> SRKTYTLTDYLKNTYRLKLYSLRWISDHEYLYKQENNILVFNAEYGNSSVFLENSTFDEFGHSINDYSISPDGQFILLEYNYVKQWRHSYTASYDIYDLNKRQLITEERIPNNTQWVTWSPVGHKLAYVWNNDIYVKIEPNLPSYRITWTGKEDIIYNGITDWVYEEEVFSAYSALWWSPNGTFLAYAQFNDTEVPLIEYSFYSDESLQYPKTVRVPYPKAGAVNPTVKFFVVNTDSLSSVTNATSIQITAPASMLIGDHYLCDVTWATQERISLQWLRRIQNYSVMDICDYDESSGRWNCLVARQHIEMSTTGWVGRFRPSEPHFTLDGNSFYKIISNEEGYRHICYFQIDKKDCTFITKGTWEVIGIEALTSDYLYYISNEYKGMPGGRNLYKIQLSDYTKVTCLSCELNPERCQYYSVSFSKEAKYYQLRCSGPGLPLYTLHSSVNDKGLRVLEDNSALDKMLQNVQMPSKKLDFIILNETKFWYQMILPPHFDKSKKYPLLLDVYAGPCSQKADTVFRLNWATYLASTENIIV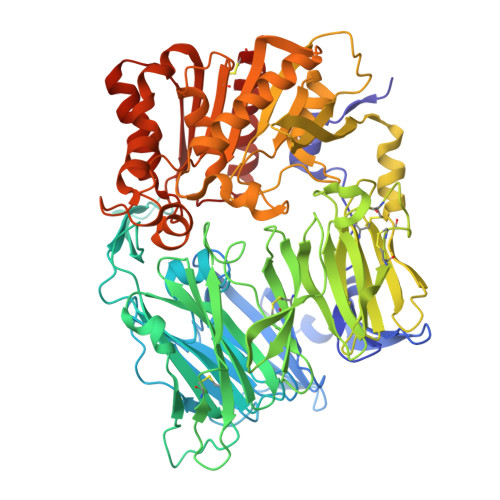ASFDGRGSGYQGDKIMHAINRRLGTFEVEDQIEAARQFSKMGFVDNKRIAIWGWSYGGYVTSMVLGSGSGVFKCGIAVAPVSRWEYYDSVYTERYMGLPTPEDNLDHYRNSTVMSRAENFKQVEYLLIHGTADDNVHFQQSAQISKALVDVGVDFQAMWYTDEDHGIASSTAHQEIYTHMSHFIKQCFSLP Butyryl Coenzyme A | C25 H42 N7 O17 P3 S 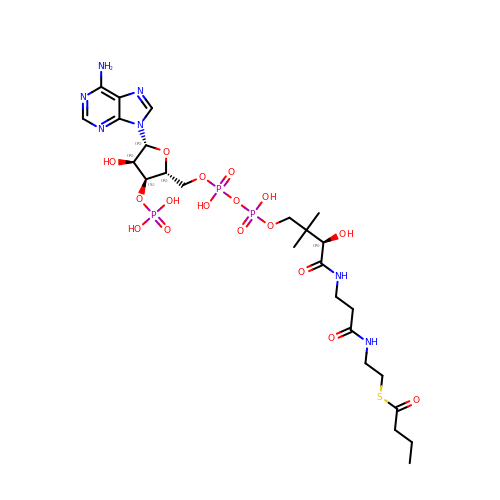| CRFNGMNYKDXRTN-CITAKDKDSA-N>LYFQGAMCYIIAKRFKKSGCVALKAKRGKELADFATDLQKKLGYDIQIVAITRPTAYGEYEPYKFVNSFEEFSIEASRL[2x];>MYILDKIGLNIEILESLSYESKLGMSFKRTLSHFNKEEVLKEIELINNWYFSLEIIDDLPLDSRIKSVSSAKMKFERYYPNATYNRVFNDILGFRVICKSYDEVLELEKEDKIRVVDMSRGKSNDDGFRGIHVYYQRDNHHYPIEIQFNTYYDRQLNDWLHDKFYKRGYDSSCGQLLRKYYENGKIKSAEELEEVLEDVLYHCKK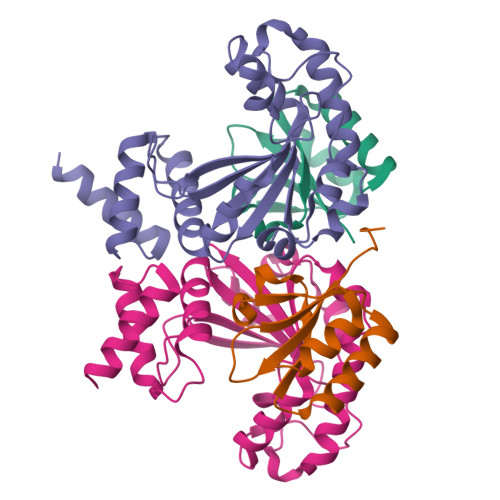I[2x]1-[3-amino-6-(3,4,5-trimethoxyphenyl)pyrazin-2-yl]piperidine-4-carboxylic 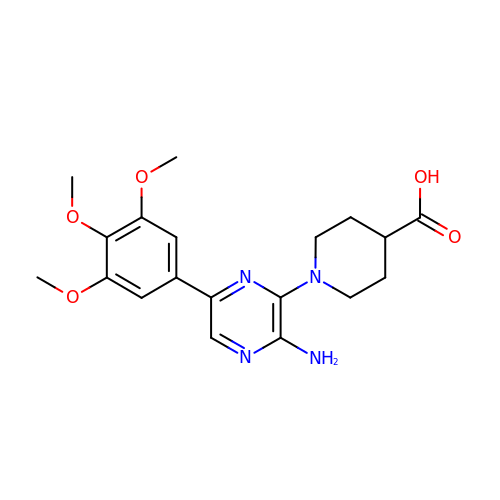acid | C19 H24 N4 O5 | FFHSQDAETWTILU-UHFFFAOYSA-N In contrast, R-spondins (Rspo1-4) are the sole secreted potentiators of Wnt signalling and have emerged as crucial regulators of stem cell maintenance in vivo and in vitro. At the level of molecular mechanism Rspo proteins potentiate Wnt signalling by alleviating the feedback inhibition effected by the transmembrane E3 ligases ZNRF3 and RNF43. Although necessary, binding of Rspo to the E3 ectodomains is not sufficient to stop ubiquitination of Frizzled and enhance Wnt signalling. This further requires simultaneous binding of Rspo to the large leucine-rich repeat (LRR) containing ectodomain of LGR receptors 4, 5 or 6, which are well established GPCR-like regulators of stem cell function. The ternary complex between Rspo and its two receptors LGR4-6 and ZNRF3/RNF43 is established via extracellular recognition and triggers by an unknown mechanism its rapid internalisation.

To obtain insight into ternary complex formation with ZNRF3 we solved a low resolution hLGR5ecto–mRspo2Fu1-Fu2–mZNRF3ecto complex. This complex is very similar to the equivalent RNF43-containing complex in the overall positioning of the three different types of subunits. The RspoFu1-Fu2 fragment is sandwiched between the two receptor ectodomains which do not contact each other. Thus, a Rspo ligand serves to heterodimerize an LGR receptor with an E3 receptor in both flavours of ternary complex. However, as previously proposed by us the ternary complex involving ZNRF3 adopts a clear 2:2:2 stoichiometry in the crystal lattice due to dimerisation of the ZNRF3 ectodomain. Compared to the relative position of RNF43 in the ternary complex, each ZNRF3 subunit is rotated 30° away from its partner LGR5. We note that dimerisation of ZNRF3ecto and consequent 2:2:2 stoichiometry of the ternary complex would not be compatible with the exact arrangement of ligand and receptors as seen in the RNF43 ternary complex due to clashes of the membrane-proximal regions of the two LGR receptors (not shown). This rigid body shift in the position of the ZNRF3/RNF43 relative to LGR also requires a re-orientation of the Rspo2Fu1 domain to maintain the β-hairpin 1 and 2 mediated interface with the E3. It appears that the difference in relative orientation of the LGR and E3 receptors for the RNF3 versus ZNRF43 ternary complex renders this flexibility a necessity for Rspo to function as a cross-linker in both contexts. Our crystallographic LGR5–Rspo–ZNRF3 complex, albeit at low resolution, confirms the 2:2:2 stoichiometry that we had hypothesised would be favoured for ternary complexes involving ZNRF3, as opposed to the 1:1:1 stoichiometry seen for the corresponding RNF43 complex.

> ETLRGCPTHCHCEPDGRMLLRVDCSDLGLSELPSNLSVFTSYLDLSMNNISQLLPNPLPSLRFLEELRLAGNALTYIPKGAFTGLYSLKVLMLQNNQLRHVPTEALQNLRSLQSLRLDANHISYVPPSCFSGLHSLRHLWLDDNALTEIPVQAFRSLSALQAMTLALNKIHHIPDYAFGNLSSLVVLHLHNNRIHSLGKKCFDGLHSLETLDLNYNNLDEFPTAIRTLSNLKELGFHSNNIRSIPEKAFVGNPSLITIHFYDNPIQFVGRSAFQHLPELRTLTLNGASQITEFPDLTGTANLESLTLTGAQISSLPQTVCNQLPNLQVLDLSYNLLEDLPSFSVCQKLQKIDLRHNEIYEIKVDTFQQLLSLRSLNLAWNKIAIIHPNAFSTLPSLIKLDLSSNLLSSFPITGLHGLTHLKLTGNHALQSLISSENFPELKVIEMPYAYQCCAFGVCENNGNNGDSVQCSPSGTHHHHHHHHHH;> ETGICKGCLSCSKDNGCSRCQQKLFFFLRREGMRQYGECLHSCPSGYYGHRAPDMNRCARCRIENCDSCFSKDFCTKCKVGFYLHRGRCFDECPDGFAPLDETMECVEGTHHHHHHHHHH;> ETGKETAFVEVVLFESSPSGDYTTHTTGLTGRFSRAGAMLSAEGEIVQMHPLGLCNNNDEEDLYEYGWVGVVKLEQPELDPKPCLTVLGKAKRAVQRGATAVIFDVSENPEAIDQLNQGSEDPLKRPVVYVKGADAIKLMNIVNKQKVARARIQHLGTKHHHHHH>VIEKVQHIQLLQKNVRAQLVDMKRLEVDIDIKIRSCRGSCSRALAREVDLKDYEDQQKQLEQVIAK[2x];>[2x]HQLYIDETVNSNIPTNLRVLRSILENLRSKIQKLESDVSAQMEYCRTPCTVSCNIPVVSGKECEEIIRKGGETSEMYLIQPDSSVKPYRVYCDMNTENGGWTVIQNRQDGSVDFGRKWDPYKQGFGNVATNTDGKNYCGLPGEYWLGNDKISQLTRMGPTELLIEMEDWKGDKVKAHYGGFTVQNEANKYQISVNKYRGTAGNALMDGASQLMGENRTMTIHNGMFFSTYDRDNDGWLTSDPRKQCSKEDGGGWWYNRCHAA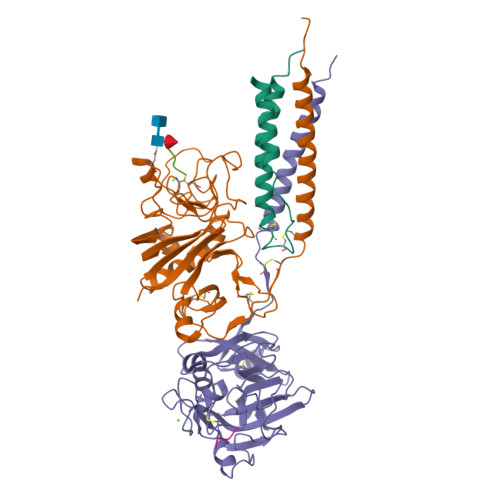NPNGRYYWGGQYTWDMAKHGTDDGVVWMNWKGSWYSMRKMSMKIRPFFPQQ;>YEASILTHDSSIRYLQEIYNSNNQKIVNLKEKVAQLEAQCQEPCKDTVQIHDITGKDCQDIANKGAKQSGLYFIKPLKANQQFLVYCEIDGSGNGWTVFQKRLDGSVDFKKNWIQYKEGFGHLSPTGTTEFWLGNEKIHLISTQSAIPYALRVELEDWNGRTSTADYAMFKVGPEADKYRLTYAYFAGGDAGDAFDGFDFGDDPSDKFFTSHKGMQFSTWDNDNDKFEGNCAEQDGSGWWMNKCHAGHLNGVYYQGGTYSKASTPNGYDNGIIWATWKTRWYSMKKTTMKIIPFNRLTIGEGQQHHLGGAK[2x];>[4x]GPRP>[4x]GPLGSGQCLYKI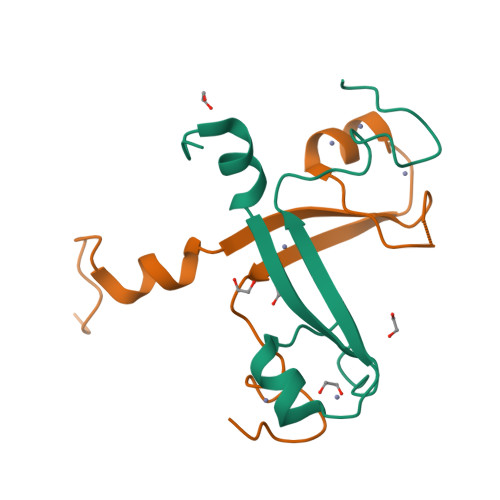SSYTSYPMHDFYRCHTCNTTDRNAICVNCIKKCHQGHDVEFIRHDRFFCDCGAGTLSNPCTLAGE>[2x]MARQVFDDKLLAVISGNSIGVLATIKHDG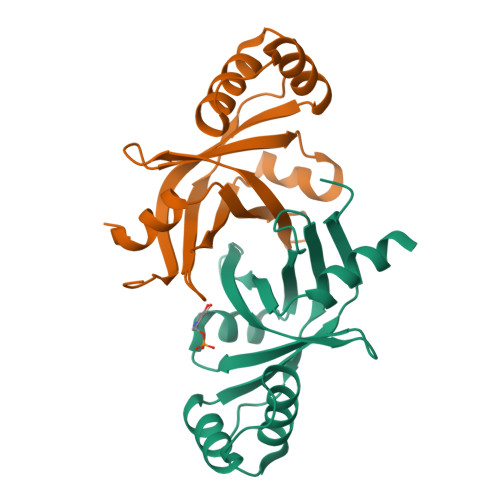RPQLSNVQYHFDPRKLLIQVSIAEPRAKTRNLRRDPRASILVDADDGWSYAVAEGTAQLTPPAAAPDDDTVEALIALYRNIAGEHSDWDDYRQAMVTDRRVLLTLPISHVYGLPPGMR5'-O-[(R)-hydroxy{[(2S)-pyrrolidin-2-ylcarbonyl]oxy}phosphoryl]adenosine 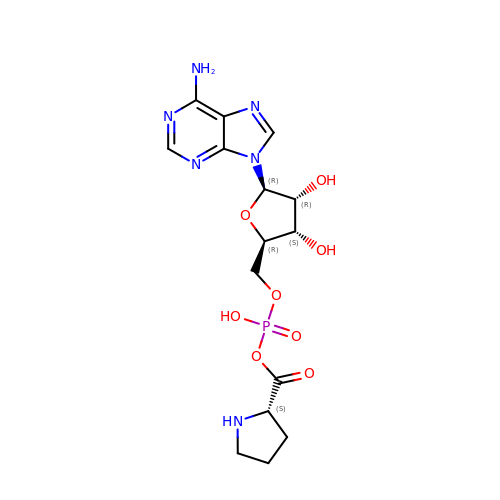| C15 H21 N6 O8 P | KQFKHTAASHMYDJ-TWBCTODHSA-N>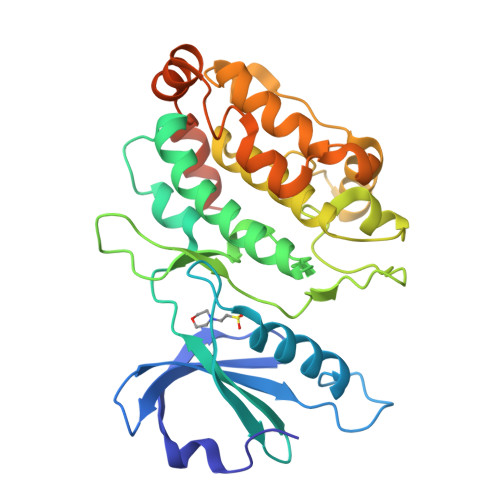 GTVFRQENVDDYYDTGEELGSGQFAVVKKCREKSTGLQYAAKFIKKRRTKSSRRGVSREDIEREVSILKEIQHPNVITLHEVYENKTDVILILELVAGGELFDFLAEKESLTEEEATEFLKQILNGVYYLHSLQIAHFDLKPENIMLLDRNVPKPRIKIIDFGLAHKIDFGNEFKNIFGTPEFVAPEIVNYEPLGLEADMWSIGVITYILLSGASPFLGDTKQETLANVSAVNYEFEDEYFSNTSALAKDFIRRLLVKDPKKRMTIQDSLQHPWIKPKDTQQALSRKASAVNMEKFKKFAARKKSNNGSGGGLNDIFEAQKIEWHE> ESARSQVQVHAPVVAARLRNIWPKFPKWLHEAPLAVAWEVTRLFMHCKVDLEDESLGLKYDPSWSTARDVTDIWKTLYRLDAFRGKPFPEKPPNDVFVTAMTGNFESKGSAVVLSAVLDYNPDNSPTAPLYLVKLKPLMFEQGCRLT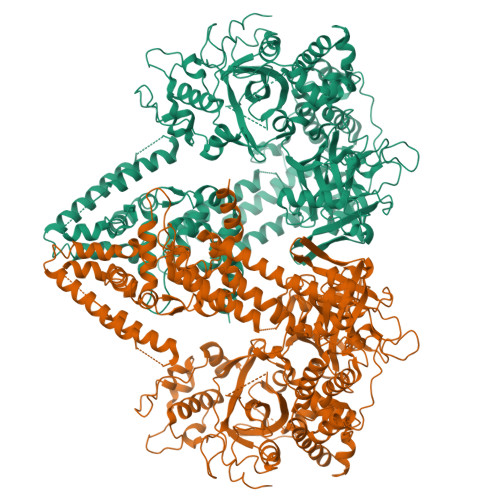RRFGPDRFFEILIPSPTSTSPSVPPVVSKQPAAVEEVIQWLTMGQHSLVGRQWRAFFAKDAGYRKPLREFQLRAEDPKPIIKERVHFFAETGITFRPDVFKTRSVVPAEEPVEQRTEFKVSQMLDWLLQLDNNTWQPHLKLFSRIQLGLSKTYAIMTLEPHQIRHHKTDLLSPSGTGEVMNDGVGRMSRSVAKRIRDVLGLGDVPSAVQGRFGSAKGMWVIDVDDTGDEDWIETYPSQRKWECDFVDKHQRTLEVRSVASELKSAGLNLQLLPVLEDRARDKVKMRQAIGDRLINDLQRQFSEQKHALNRPVEFRQWVYESYSSRATRVSHGRVPFLAGLPDSQEETLNFLMNSGFDPKKQKYLQDIAWDLQKRKCDTLKSKLNIRVGRSAYIYMIADFWGVLEENEVHVGFSSKFRDEEESFTLLSDCDVLVARSPAHFPSDIQRVRAVFKPELHSLKDVIIFSTKGDVPLAKKLSGGDYDGDMAWVCWDPEIVDGFVNAEMPLEPDLSRYLKKDKTTFKQLMASHGTGSAAKEQTTYDMIQKSFHFALQPNFLGMCTNYKERLCYINNSVSNKPAIILSSLVGNLVDQSKQGIVFNEASWAQLRRELLGGALSLPDPMYKSDSWLGRGEPTHIIDYLKFSIARPAIDKELEAFHNAMKAAKDTEDGAHFWDPDLASYYTFFKEISDKSRSSALLFTTLKNRIGEVEKEYGRLVKNKEMRDSKDPYPVRVNQVYEKWCAITPEAMDKSGANYDSKVIRLLELSFLADREMNTWALLRASTAFKLYYHKSPKFVWQMAGRQLAYIKAQMTSRPGEGAPALMTAFMYAGLMPDKKFTKQYVARLEGDGSEYPDPEVYEVLGDDDFDGIGFTGNGDY>MHHHHHHENLYFQGAA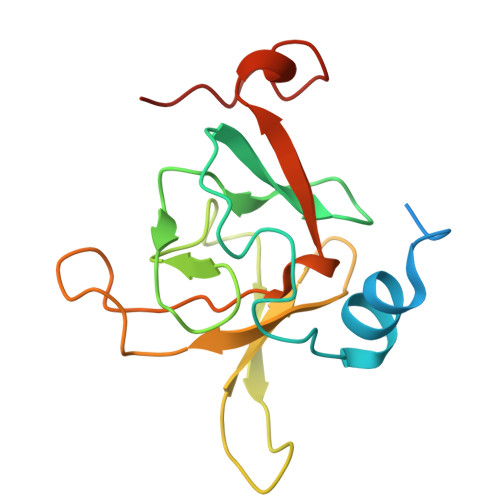SMLKKDKSELTDIEYIVTQENGTEPPFMNEYWNHFAKGIYVDKISGKPLFTSEEKFHSECGWPSFSKALDDDEIIELVDKSFGMVRTEVRSEESNSHLGHVFNDGPKESGGLRYCINSAAIQFIPYEKLEELGYGDLISHFDK[6x]(3S,11E)-14,16-dihydroxy-3-methyl-3,4,5,6,9,10-hexahydro-1H-2-benzoxacyclotetradecine-1,7(8H)-dione | C18 H22 O5 | 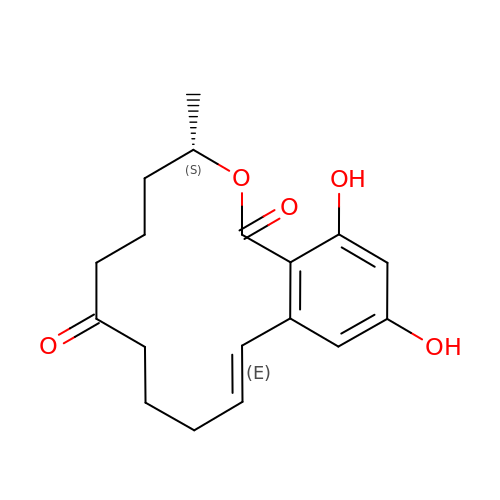MBMQEIFVQACCCH-QBODLPLBSA-N> MNVYDDVLDATVVSHSLATHFTTSDYEELLVVRTNILSVYRPTRDGKLYLTDEFKFHGLITDIGLIPQKDSPLSCLLLCTGVAKISILKFNTLTNSIDTLSLHYYEGKFKGKSLVELAKISTLRMDPGSSCALLFNNDIIAFLPFHVNKNDDDEEEEDEDENIDDSELIHSMNQKSQGTNTFNKRKRTKLGDKFTAPSVVLVASELYEGAKNIIDIQFLKNFTKPTIALLYQPKLVWAGNTTISKLPTQYVILTLNIQPAESATKIESTTIAFVKELPWDLHTIVPVSNGAIIVGTNELAFLDNTGVLQSTVLLNSFADKELQKTKIINNSSLEIMFREKNTTSIWIPSSKSKNGGSNNDETLLLMDLKSNIYYIQMEAEGRLLIKFDIFKLPIVNDLLKENSNPKCITRLNATNSNKNMDLFIGFGSGNALVLRLNNLKSTIETREAHNPSSGTNSLMDINDDDDEEMDDLYADEAPENGLTTNDSKGTVETVQPFDIELLSSLRNVGPITSLTVGKVSSIDDVVKGLPNPNKNEYSLVATSGNGSGSHLTVIQTSVQPEIELALKFISITQIWNLKIKGRDRYLITTDSTKSRSDIYESDNNFKLHKGGRLRRDATTVYIS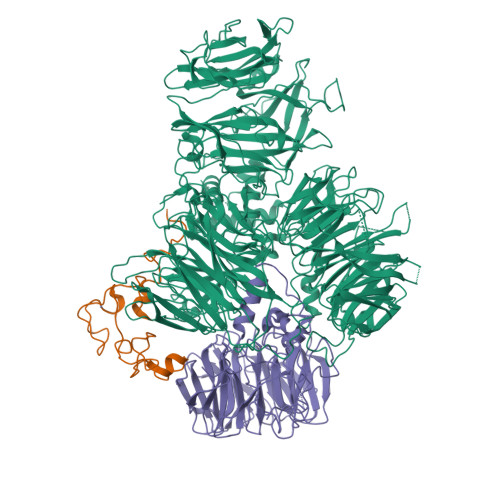MFGEEKRIIQVTTNHLYLYDTHFRRLTTIKFDYEVIHVSVMDPYILVTVSRGDIKIFELEEKNKRKLLKVDLPEILNEMVITSGLILKSNMCNEFLIGLSKSQEEQLLFTFVTADNQIIFFTKDHNDRIFQLNGVDQLNESLYISTYQLGDEIVPDPSIKQVMINKLGHDNKEEYLTILTFGGEIYQYRKLPQRRSRFYRNVTRNDLAITGAPDNAYAKGVSSIERIMHYFPDYNGYSVIFVTGSVPYILIKEDDSTPKIFKFGNIPLVSVTPWSERSVMCVDDIKNARVYTLTTDNMYYGNKLPLKQIKISNVLDDYKTLQKLVYHERAQLFLVSYCKRVPYEALGEDGEKVIGYDENVPHAEGFQSGILLINPKSWKVIDKIDFPKNSVVNEMRSSMIQINSKTKRKREYIIAGVANATTEDTPPTGAFHIYDVIEVVPEPGKPDTNYKLKEIFQEEVSGTVSTVCEVSGRFMISQSQKVLVRDIQEDNSVIPVAFLDIPVFVTDSKSFGNLLIIGDAMQGFQFIGFDAEPYRMISLGRSMSKFQTMSLEFLVNGGDMYFAATDADRNVHVLKYAPDEPNSLSGQRLVHCSSFTLHSTNSCMMLLPRNEEFGSPQVPSFQNVGGQVDGSVFKIVPLSEEKYRRLYVIQQQIIDRELQLGGLNPRMERLANDFYQMGHSMRPMLDFNVIRRFCGLAIDRRKSIAQKAGRHAHFEAWRDIINIEFSMRSLCQGK;> PSLIHPDTAKYPFKFEPFLRQEYSFSLDPDRPICEFYNSREGPKSCPRGPLCPKKHVLPIFQNKIVCRHWLRGLCKKNDQCEYLHEYNLRKMPECVFFSKNGYCTQSPDCQYLHIDPASKIPKCENYEMGFCPLGSSCPRRHIKKVFCQRYMTGFCPLGKDECDMEHPQFIIPDEGSKLRIKRDDEINTRKMDEEKERRLNAIINGEV;> MDGHNQNQYQNQNQIQQSQQPPLKKYVTQRRSVDVSSPYINLYYNRRHGLPNLVVEPETSYTIDIMPPNAYRGRDRVINLPSKFTHLSSNKVKHVIPAIQWTPEGRRLVVATYSGEFSLWNASSFTFETLMQAHDSAVTTMKYSHDSDWMISGDADGMIKIWQPNFSMVKEIDAAHTESIRDMAFSSNDSKFVTCSDDNILKIWNFSNGKQERVLSGHHWDVKSCDWHPEMGLIASASKDNLVKLWDPRSGNCISSILKFKHTVLKTRFQPTKGNLLMAISKDKSCRVFDIRYSMKELMCVRDETDYMTLEWHPINESMFTLACYDGSLKHFDLLQNLNEPILTIPYAHDKCITSLSYNPVGHIFATAAKDRTIRFWTRARPIDPNAYDDPTYNNKKINGWFFGINNDINAVREKSEFGAAPPPPATLEPHALPNMNGFINKKPRQEIPGIDSNIKSSTLPGLSIXXXXX> KEELDKLDYFELFKEYLKKREENHEKLLKILDELLDEVKK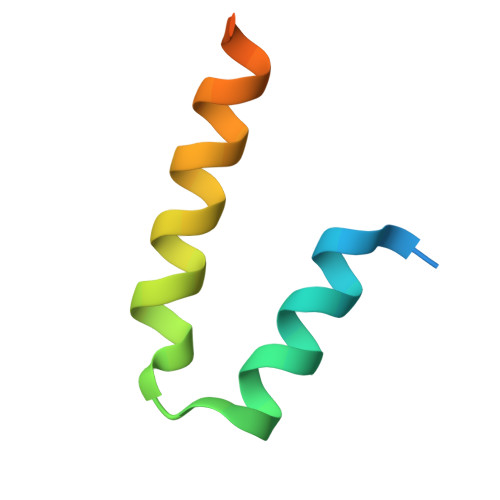SEAGHHHHHH>[2x]TEVDPTHFEKRFLKRIRDLGEGHFGKVELCRYDPEGDNTGEQVAVKSLKPESGGNHIADLKKEIEILRNLYHENIVKYKGICTEDGGNGIKLIMEFLPSGSLKEYLPKNKNKINLKQQLKYAVQICKGMDYLGSRQYVHRDLAARNVLVESEHQVKIGDFGLTKAIETDKEYYTVKDDRDSPV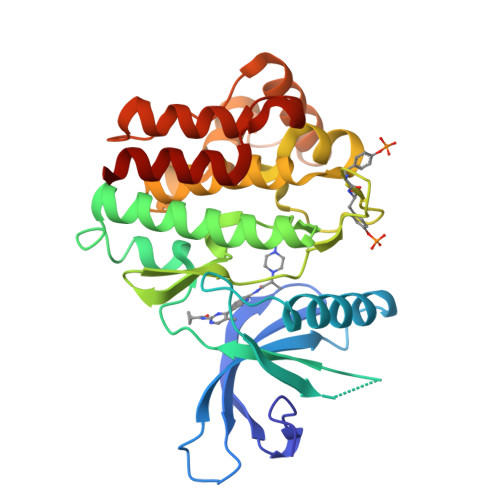FWYAPECLMQSKFYIASDVWSFGVTLHELLTYCDSDSSPMALFLKMIGPTHGQMTVTRLVNTLKEGKRLPCPPNCPDEVYQLMRKCWEFQPSNRTSFQNLIEGFEALLK> LNSDGLTLLSLLKHLDRVPPQVTSTWKINASEATPCNWFGITCDDSKNVASLNFTRSRVSGQLGPEIGELKSLQILDLSTNNFSGTIPSTLGNCTKLATLDLSENGFSDKIPDTLDSLKRLEVLYLYINFLTGELPESLFRIPKLQVLYLDYNNLTGPIPQSIGDAKELVELSMYANQFSGNIPESIGNSSSLQILYLHRNKLVGSLPESLNLLGNLTTLFVGNNSLQGPVRFGSPNCKNLLTLDLSYNEFEGGVPPALGNCSSLDALVIVSGNLSGTIPSSLGMLKNLTILNLSENRLSGSIPAELGNCSSLNLLKLNDNQLVGGIPSALGKLRKLES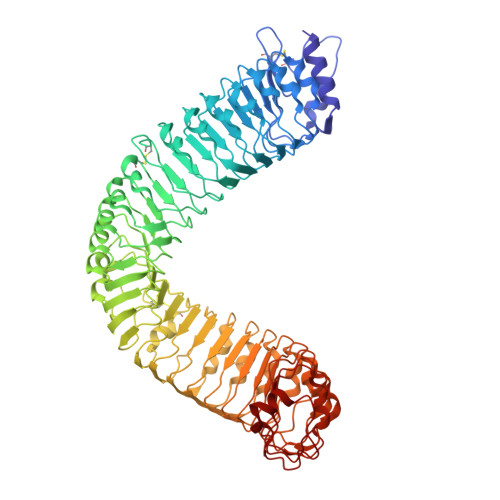LELFENRFSGEIPIEIWKSQSLTQLLVYQNNLTGELPVEMTEMKKLKIATLFNNSFYGAIPPGLGVNSSLEEVDFIGNKLTGEIPPNLCHGRKLRILNLGSNLLHGTIPASIGHCKTIRRFILRENNLSGLLPEFSQDHSLSFLDFNSNNFEGPIPGSLGSCKNLSSINLSRNRFTGQIPPQLGNLQNLGYMNLSRNLLEGSLPAQLSNCVSLERFDVGFNSLNGSVPSNFSNWKGLTTLVLSENRFSGGIPQFLPELKKLSTLQIARNAFGGEIPSSIGLIEDLIYDLDLSGNGLTGEIPAKLGDLIKLTRLNISNNNLTGSLSVLKGLTSLLHVDVSNNQFTGPIPDNLEGQLLSEPSSFSGNPNLCIP>[4x]MSLKNKLQVKIPGKLYVAGEYAVVESGH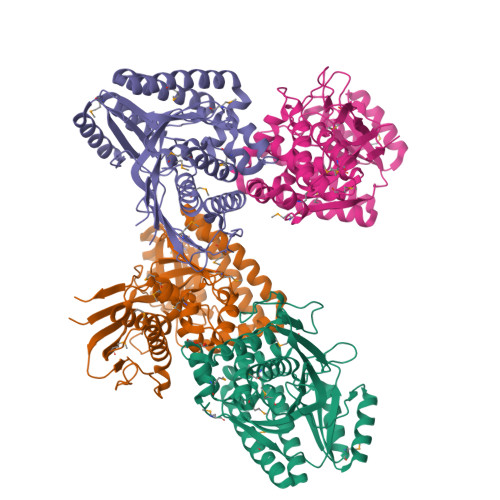TAILTAVNRYITLTLEDSERNELWIPHYENPVSWPIGGELKPDGEHWTFTAEAINIATTFLKSEGIELTPVKMVIETELIDQSGAKYGLGSSAAATVAVINALMTKFYPEISMLKKFKLAALSHLVVQGNGSCGDIASCMYGGWIAYTTFDQEWVKHRLAYKSLEWFMKEPWPMLQIETLEEPVPTFSVGWTGTPVSTGKLVSQIHAFKQEDSKNYQHFLTRNNEIMKQIIQAFHTKDEELLYSSIKENRRILQELGTKAGVNIETSLLKELADSAENMGGAGKSSGSGGGDCGIAFSKTKELAEKLVNEWEKLGIKHLPFHTGRVQITEGHHHHHH>[6x]TQTLPAEGEIGLIDVGSLQLESGAVIDDVCIAVQRWGKLSPARDNVVVVLHALTGDSHITGPAGPGHPTPGWWDGVAGPGAPIDTTRWCAVATNVLGGCRGSTGPSSLARDGKPWGSRFPLISI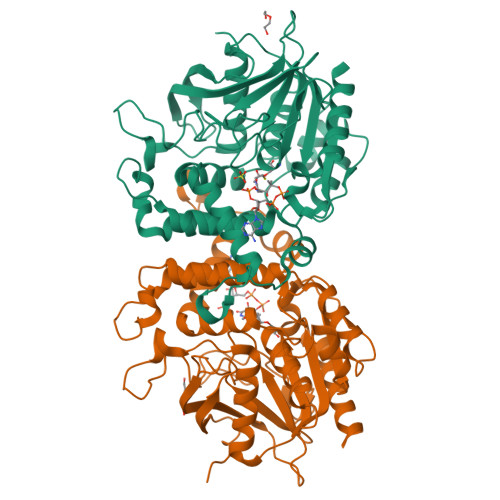RDQVQADVAALAALGITEVAAVVGGSMGGARALEWVVGYPDRVRAGLLLAVGARATADQIGTQTTQIAAIKADPDWQSGDYHETGRAPDAGLRLARRFAHLTYRGEIELDTRFANHNQGNEDPTAGGRYAVQSYLEHQGDKLLSRFDAGSYVILTEALNSHDVGRGRGGVSAALRACPVPVVVGGITSDRLYPLRLQQELADLLPGCAGLRVVESVYGHDGFLVETEAVGELIRQTLGLADREG[(2~{R},3~{S},5~{R})-5-[(4~{E})-4-hydroxyimino-2-oxidanylidene-1,3-diazinan-1-yl]-3-oxidanyl-oxolan-2-yl]methyl 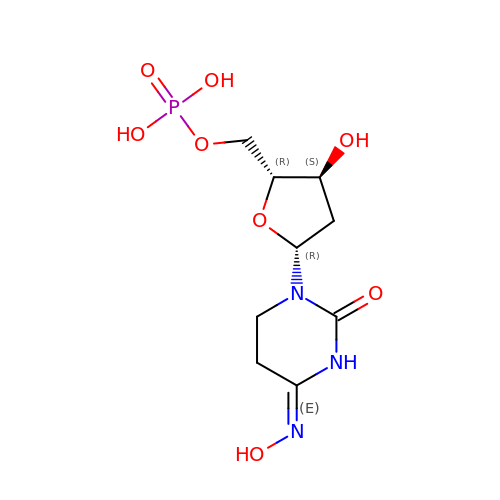dihydrogen phosphate | C9 H16 N3 O8 P | BXCKTJBMNGLVHU-SHYZEUOFSA-N Here, the first crystal structures from PF02663 are described, representing two bacterial and one archaeal species: B8FYU2_DESHY from the anaerobic dehalogenating bacterium Desulfito­bacterium hafniense DCB-2, Q2LQ23_SYNAS from the syntrophic bacterium Syntrophus aciditrophicus SB and Q9HJ63_THEAC from the thermoacidophilic archaeon Thermoplasma acidophilum. Two of these proteins, Q9HJ63_THEAC and Q2LQ23_SYNAS, contain two domains: an N-terminal thioredoxin-like α+β core domain (NTD) consisting of a five-stranded, mixed β-sheet flanked by several α-helices and a C-terminal zinc-finger domain (CTD). The proximity of fmdE to genes encoding the catalytic subunits suggests a role in methanogenesis for proteins in PF02663. Individual proteins within this family display differences in domain architectures, metal-ion binding propensities and dimer interactions.

Molecular replacement was then used to determine the structure of the I222 crystal form at 1.87 Å resolution. The final model includes one protein molecule (residues 1–201), one unknown ligand (UNL), five Zn atoms, six ethylene glycol molecules, eight acetate ions and 129 water molecules in the asymmetric unit. All three crystal forms show zinc binding at the same two sites, suggesting that these sites are functionally relevant (note that two of the three crystal forms, C2 and P42212, are devoid of exogenous zinc in the crystallization conditions). The I222 crystal form also showed four additional zinc-binding sites, which are likely to be attributable to the presence of zinc acetate in the crystallization experiments. In Q9HJ63_THEAC the zinc-binding site on the NTD is situated on a loop connecting the N-terminal α-helices (α1 and α2). The UNL is only 1.8 Å from the S atom of the conserved Cys61, which is consistent with a thioester bond between the protein and the UNL. Two significant structural differences between Q9HJ63_THEAC and Q2LQ23_SYNAS involve their metal binding. First, zinc is bound to the putative active site on the NTD of Q9HJ63_THEAC, but is absent from the NTD of Q2LQ23_SYNAS. Second, whereas the structure of the CTD of Q2LQ23_SYNAS shows four Cys side chains within coordination distance of the Zn atom, the structure of Q9HJ63_THEAC is atypical for a treble-cleft zinc finger in that three Cys side chains and an Asp side chain are within coordination distance of the zinc. A FATCAT search of the PDB shows that the structure of the zinc-finger CTD on Q9HJ63_THEAC is similar to the individual treble-clef zinc-finger subdomains of several eukaryotic LIM-like proteins.

> GMEKLNFGIPEWAFEFHGHKCPYMPMGYRAGSYALKIAGLEKEKDHRTYLLSEMSPEDMNGCFNDGAQAATGCTYGKGLFSLLGYGKLALILYRPGRKAIRVHVRNSFMDELSTRASDFFRYRKQGYEPSEIPAGAIDPVLEWISSLEDEEIFEYREIDGFTFEPVKKNGAKVRCDVCGEYTYEADAKLLNGKPVCKPDYYGKK> MGYVGIKIRLTDVAPQAQELFKKESLDVKENKVYLVAATLRPETMYGQTCCFVSPKIDYGVFDAGNGDYFITTERAFKNMSFQNLTPKRGYYKPLFTINGKTLIGSRIDAPYAVNKNLRVLPMETVLATKGTGVVTCVPSDSPDDF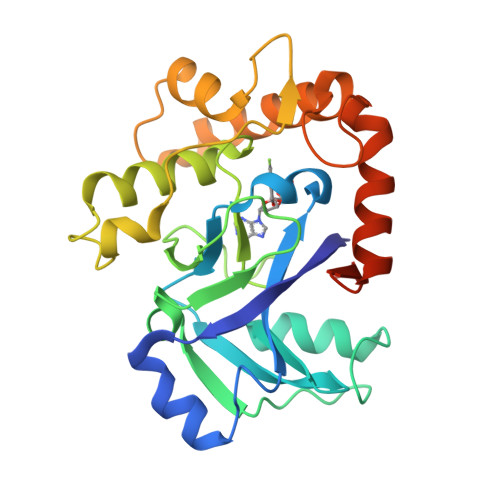VTTRDLANKPEYYGIEKDWVQTDIVPIVHTEKYGDKCAEFLVNDLKIQSPKDSVQLANAKELAYKEGFYNGTMLIGKYKGDKVEDAKPKVKQDLIDEGLAFVYDEPELEHHHHHH>[2x]MNEKYVVTWDMLQIHARKLAQRLLPAEQWKGIIAVSRGGLVPAGILARELGIR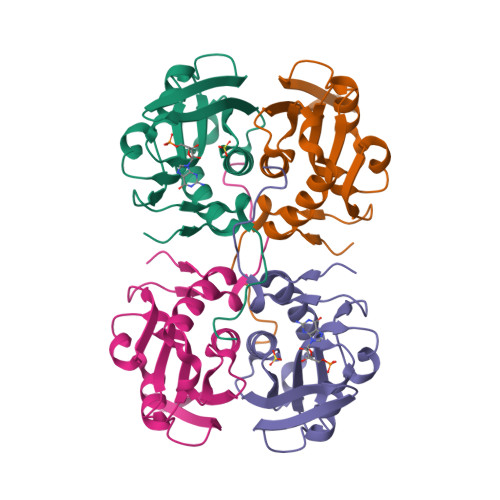YVDTVCISSYDHDNQRDLKVLKRAEGDGEGFIVIDDLVDTGGTATAIREMYPKAHFVTIFAKPAGRPLVDDYVVDIPQNTWIEQPWDMAVTFVAPLSGK>SENLKDEILEKYIPKTKKTRSGHIVIKTEETPNPEIVANTRTVPGIITARGCAYAGCKGVVMGPIKDMVHITHGPIGCSFYTWGGRRFKSKPENGTGLNFNEYVFSTDMQESDIVFGGVNKLKDAIHEAYEMFHPAAIGVYATCPVGLIGDDILAVAATASKEIGIPVHAFSCEGYKGVSQSAGHHIANNTVMTDIIGKGNKEQKKYSINVLGEYNIGGDAWEMDRVLEKIGYHVNATLTGDATYEKVQNADKADLNLVQCHRSINYIAEMMETKYGIPWIKCNFIGVDGIVETLRDMAKCFDDPELTKRTEEVIAEEIAAIQDDLDYFKEKLQGKTACLYVGGSRSHTYMNMLKSFGVDSLVAGFEFAHRDDYEGREVIPTIKIDADSKNIPEITVTPDEQKYRVVIPEDKVEELKKAGVPLSSYGGMMKEMHDGTILIDDMNHHDMEVVLEKLKPDMFFAGIKEKFVIQKGGVLSKQLHSYDYNGPYAGFRGVVNFGHELVNGIYTPAWKMITPPWKKASSESKVVVGGEA[2x];>MLDATPKEIVERKALRINPAKTCQPVGAMYAALGIHNCLPHSHGSQGCCSYHRTVLSRHFKEPAMASTSSFTEGASVFGGGSNIKTAVKNIF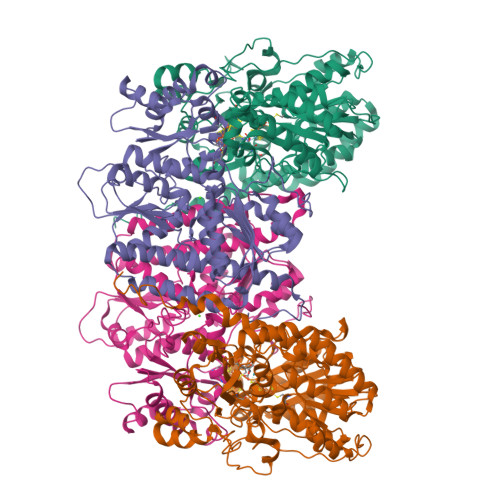SLYNPDIIAVHTTCLSETLGDDLPTYISQMEDAGSIPEGKLVIHTNTPSYVGSHVTGFANMVQGIVNYLSENTGAKNGKINVIPGFVGPADMREIKRLFEAMDIPYIMFPDTSGVLDGPTTGEYKMYPEGGTKIEDLKDTGNSDLTLSLGSYASDLGAKTLEKKCKVPFKTLRTPIGVSATDEFIMALSEATGKEVPASIEEERGQLIDLMIDAQQYLQGKKVALLGDPDEIIALSKFIIELGAIPKYVVTGTPGMKFQKEIDAMLAEAGIEGSKVKVEGDFFDVHQWIKNEGVDLLISNTYGKFIAREENIPFVRFGFPIMDRYGHYYNPKVGYKGAIRLVEEITNVILDKIERECTEEDFEVVR[2x]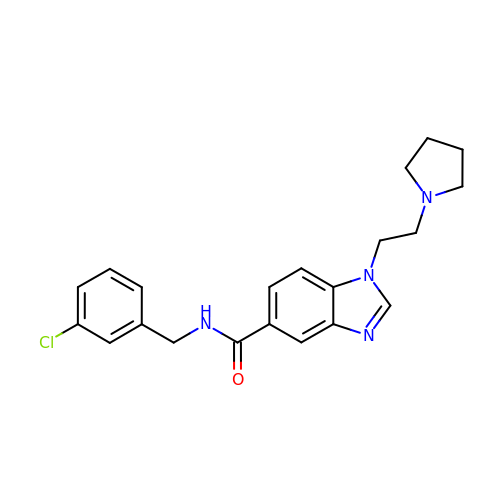~{N}-[(3-chlorophenyl)methyl]-1-(2-pyrrolidin-1-ylethyl)benzimidazole-5-carboxamide | C21 H23 Cl N4 O | KDORBCZWJTXUAC-UHFFFAOYSA-N> SGKRKLITSEEERSPAK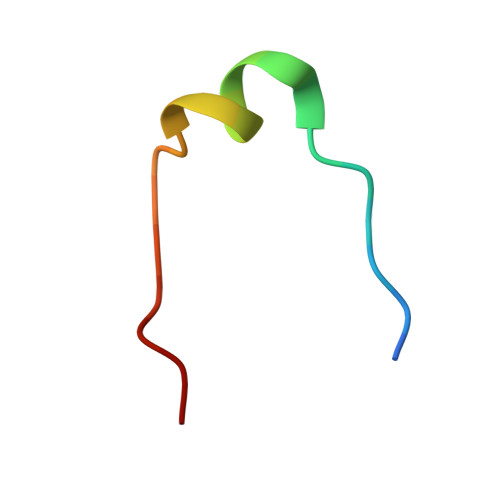RGRKS> LQELESFVGSALRTYRLLRPHALPFYKEDSLLSMQSKLNEATLKHSPLVHDLVELKKRNLSVPSDLLPPDFNALQFSLPVVSARGFLLALSAAANSVAEDLEFLCRRLSVPNLPHPTHPFRLKLLLDALFESFKLRKDPHYAHDWAQRNWPRLQAAMPEPLSELSADSVGLWLKAHLERVIENQRGRHADGRGRLLAQKFPLKSDEEDLYSLADDFIFDHEIVDEQFCDERLSQFPIDKAGELFRRVADFFGLTKGPQPAVNDAVVAQFQNLVYTLDEIGLSNWMKMDTREIEEFLPEGDPPSFAASQQDLDAARLLLKAAARGKANLLDFEALDPYKLLHGFDFKTVQEELATLPPNPFLTDADIDELFDITTAAVSMNQSEVAP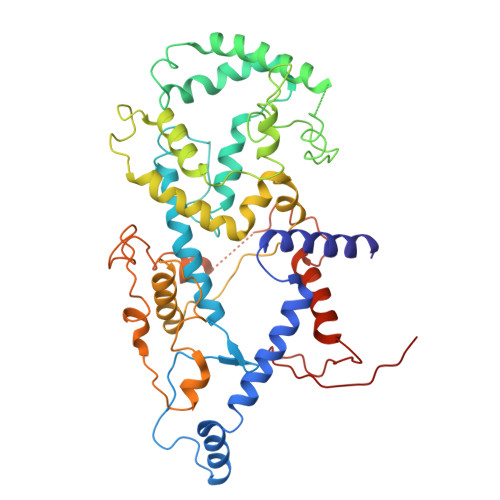SASLRNFKAKFGRTPLEALLDSEEKFLTSAGPVDWLKDEDENGEAFVSWRWKRPA>[2x]GRGSAGYDLNAFTFDPIKESIVSREMTRRYMTDMITYAETDVVVVGAGSAGLSAAYEISKNPNVQVAIIEQSVSPGGGAWLGGQLFSAMIVRKPAHLFLDEIGVAYDEQDTYVVVKHAALFTSTIMSKLLARPNVKLFNAVAAEDLIVKGNRVGGVVTNWALVAQNHHTQSCMDPNVMEAKIVVSSCGHDGPFGATGVKRLKSIGMIDHVPGMKALDMNTAEDAIVRLTR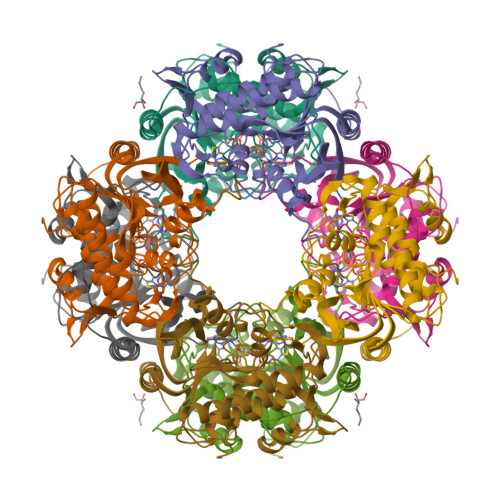EVVPGMIVTGMEVAEIDGAPRMGPTFGAMMISGQKAGQLALKALGLPNAIDGTL> GHMSKSDYIQNMFQTKSFVDRYKYTEKLTGLYAQT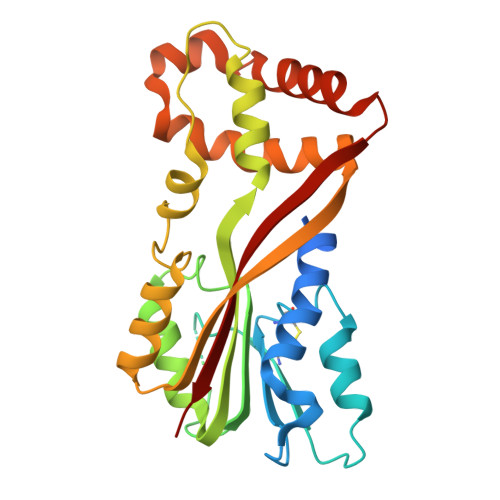LVDYSGVANTSQKPLIVLDNACGIGAVSSVLNHTLQDEAKKTWKLTCGDLSEGMLETTKRRLQDEGWVNAETKIVNALDTGLPDGHYTHVFVAFGFQSFPDANAALKECFRILASGGILASSTWQNFNWIPIMKAAIETIPGNLPFPTQKEFIALHNAGWDSESYIQSELEKLGFRDVKVIPVPKETSIPIDEFFEVCMMIIPYLLPKFWTEEQRESHEKDVPMVLRQYLQDTYGANGQVPLEAVALITTGLKP>GQDMVSPPPPIADEPLTVNTGIYLIECYSLDDKAETFKVNAFLSLSWKDRRLAFDPVRSGVRVKTYEPEAIWIPEIRFVNVENARDADVVDISVSPDGTVQYLERFSARVLSPLDFRRYPFDSQTLHIYLIVRSVDTRNIVLAVDLEKVGKNDDVFLTGWDIESFTAVVKPANFALEDRLESKLDYQLRISRQYFSYIPNIILPMLFILFISWTAFWSTSYEANVTLVVSTLIAHIAFNILVGTNLPKTPYMTYTGAIIFMIYLFYFVAVIEV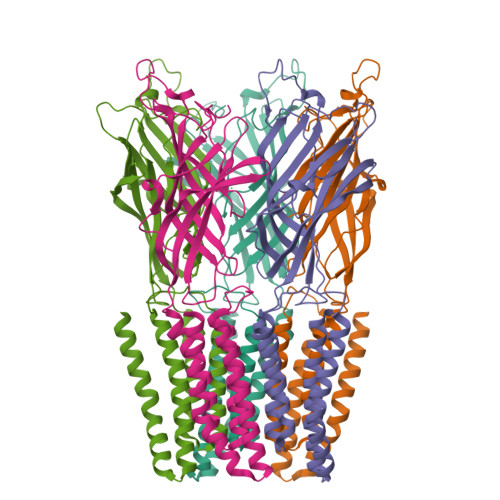TVQHYLKVESQPARAASITRASRIAFPVVFLLANIILAFLFFGF[5x]> FS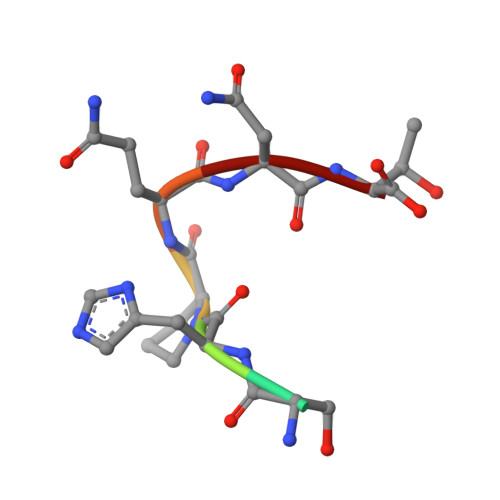HPQNT>MAHHHHHHMKVGLVGWRGMVGSVLMQRMVEENDFAHIEPFYFSTSNAGGEAPSFGGKTAPALMEATDITSLKQMDVIITCQGGDYTSEVFPKLKATGWDGYWIDAASTLRMTDDAIIVLDPVNLNVIKDGLAKGTKTFVGGNCTVSLMLMGVGALFQNNLVEWMTAMTYQAASGAGAQNMRELLTGMGYLYNNTKTLLDDPKSAILDIDRQV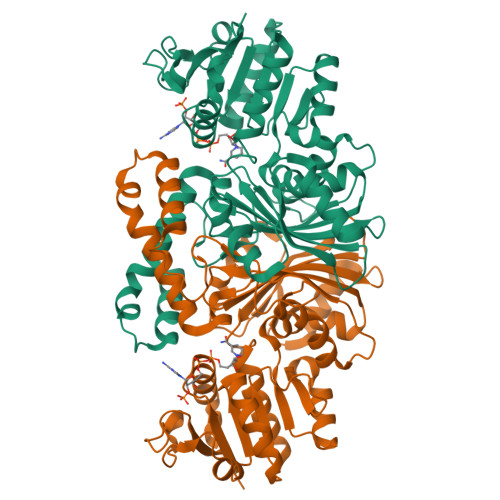AELQRGEGFPSANFGVPLAGSLIPYIDKQLESGQSKEEWKGQVETNKILGNSQIVPIDGHCVRIGAMRCHSQALTIKLKKDVPLDEIEDMIRNSNQWAKVVPNTREASMTDLTPVAVTGTLTVPVGRLRKLNMGKEYLGAFTVGDQLLWGAAEPLRRMLRILVEYKSS[2x]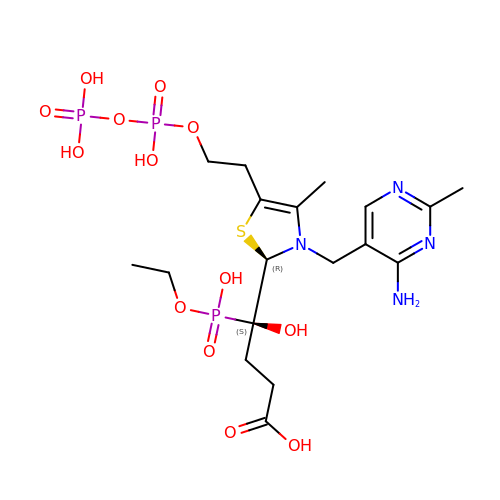(4~{S})-4-[(2~{R})-3-[(4-azanyl-2-methyl-pyrimidin-5-yl)methyl]-4-methyl-5-[2-[oxidanyl(phosphonooxy)phosphoryl]oxyethyl]-2~{H}-1,3-thiazol-2-yl]-4-[ethoxy(oxidanyl)phosphoryl]-4-oxidanyl-butanoic acid | C18 H31 N4 O13 P3 S | XUQXUYTXDQCESE-MSOLQXFVSA-N3-bromanyl-N-[5-[[3-(dimethylamino)phenyl]sulfamoyl]-1,3,4-thiadiazol-2-yl]benzamide 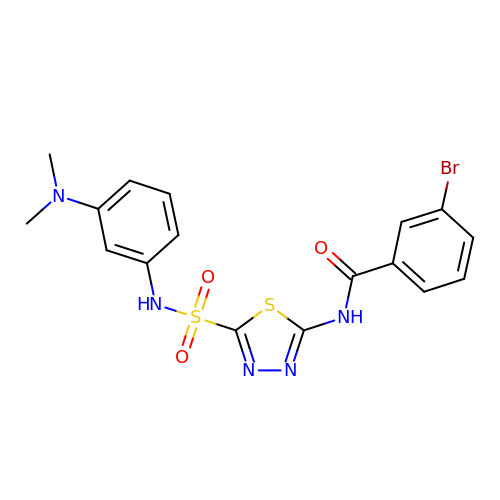| C17 H16 Br N5 O3 S2 | VAOGVNRLMMLBMF-UHFFFAOYSA-N(4-hydroxy-3,5-dimethylphenyl)(2-methyl-1-benzofuran-3-yl)methanone 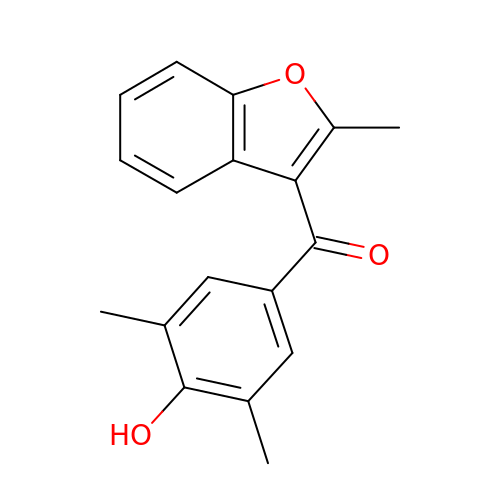| C18 H16 O3 | CIXADHNQIHMLIL-UHFFFAOYSA-N N-[(6-BUTOXYNAPHTHALEN-2-YL)SULFONYL]-D-GLUTAMIC ACID | C19 H23 N O7 S | 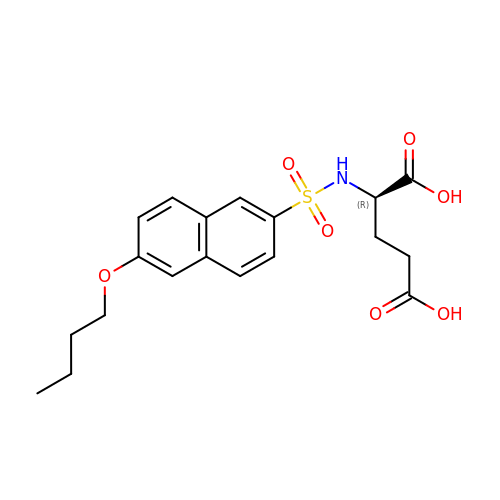UAGYXJBYAFGRFR-QGZVFWFLSA-N>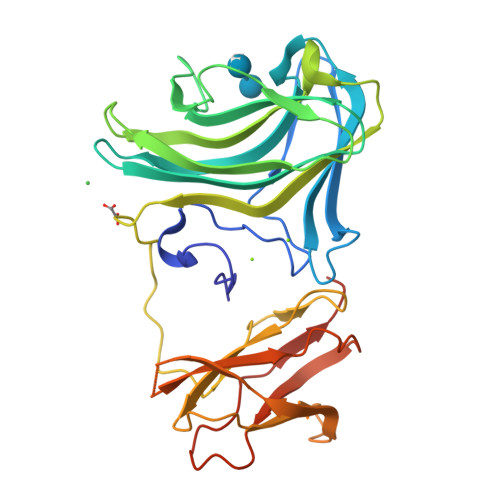 MLEDNSSTLPPYKNDLLYERTFDEGLCYPWHTCEDSGGKCSFDVVDVPGQPGNKAFAVTVLDKGQNRWSVQMRHRGLTLEQGHTYRVRLKIWADASCKVYIKIGQMGEPYAEYWNNKWSPYTLTAGKVLEIDETFVMDKPTDDTCEFTFHLGGELAATPPYTVYLDDVSLYDPEYTKPVEYILPQPDVRVNQVGYLPEGKKVATVVCNSTQPVKWQLKNAAGVVVLEGYTEPKGLDKDSQDYVHWLDFSDFATEGIGYYFELPTVNSPTNYSHPFDIRKDILEHHHHHH> GSSVVVDTNGQPVSNGADAYYLVPVSHGHAGLALAKIGNEAEPRAVVLDPHHRPGLPVRFESPLDINIIKESYFLNIKFGPSSSDSGVWDVIQQDPIGLAVKVTDTKSLLGPFKVEKEGEGYKIVYYPERGQTGLDIGLVHRNDKYYLAV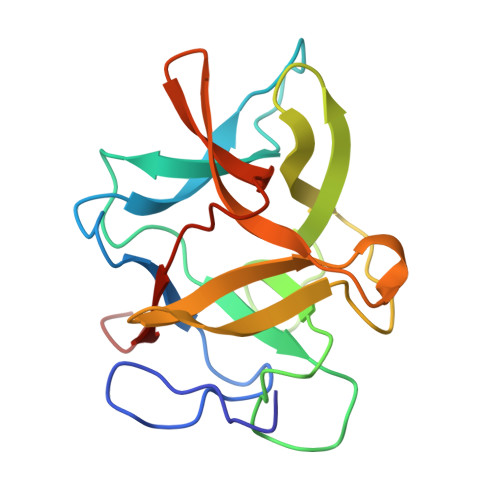KDGEPCVFKIRKATDE>[2x]MTPKKNISKGAVLHEKPMTVMVLTATEPFNYKEGKENMFHATVATES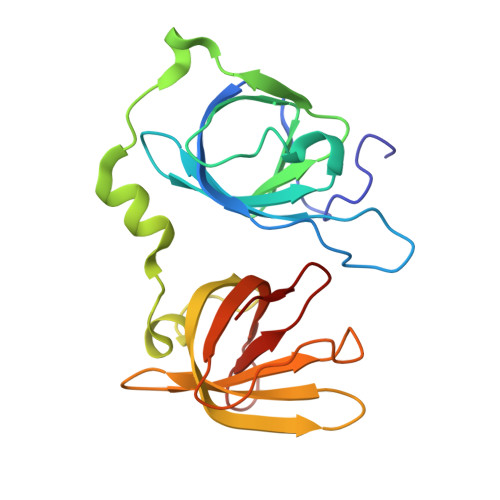QYYRVKVFNMDLKEKFTENKFITISKYFNSSGILEINETATVSEAAPNQMFEVPKNIIRSAKETLKISKIKELDSGTLIYGVFAVEKKKVNDKSITFKIKDNEDNIKVVWDKEQHNINYEKGDKLQLFSFHLRKGNGKPILHSGNHSFIKG>MQWSGARALEALLTVAGELRGPPLQLDTGQLLKIAKRGGVTAVEAVHAWRNALTGAPLNLTPEQVVAIASHDGGKQALETVQRLLPVLCQAHGLTPQQVVAIASHDGGKQALETVQRLLPVLCQAHGLTPEQVVAIASHDGGKQALETVQALLPVLCQAHGLTPEQVVAIASNGGGKQALETVQRLLPVLCQAHGLTPQQVVAIASNGGGKQALETVQRLLPVLCQAHGLTPQQVVAIASRGGKQALETVQRLLPVLCQAHGLTPQQVVAIASNNGGKQALETVQRLLPVLCQAHGLTPQQVVAIASHDGGKQALETVQRLLPVLCQAHGLTPQQVVAIASNNGGKQALETVQRLLPVLCQAHGLTPEQVVAIASNGGGKQALETVQRLLPVLCQAHGLTPEQVVAIASHDGGKQALETVQRLLPVLCQAHGLTPQQVVAIASNGG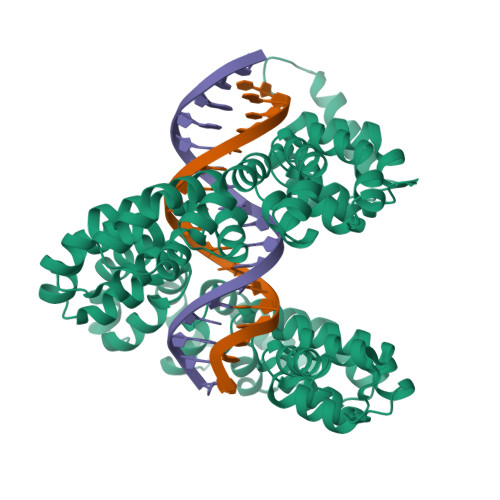GRPALESIVAQLSRPDPALAALTNDHLVALACLGGRPALDAVKKLEHHHHHH[2x]> MDEAVGDLKQALPCVAESPTVHVEVHQRGSSTAKKEDINLSVRKLLNRHNIVFGDYTWTEFDEPFLTRNVQSVSIIDTELKVKDSQPIDLSACTVALHIFQLNEDGPSSENLEEETENIIAANHWVLPAAEFHGLWDSLVYDVEVKSHLLDYVMTTLLFSDKNVNSNLITWNRVVLLHGPPGTGKTSLCKALAQKLTIRLSSRYRYGQLIEINSHSLFSKWFSESGKLVTKMFQKIQDLIDDKDALVFVLIDAVESLTAARNACRAGTEPSDAIRVVNAVLTQIDQIKRHSNVVILTTSNITEKIDVAFVDRADIKQYIGPPSAAAIFKIYLSCLEELMKCQIIYPRQQLLTLRELEMIGFIENNVSKLSLL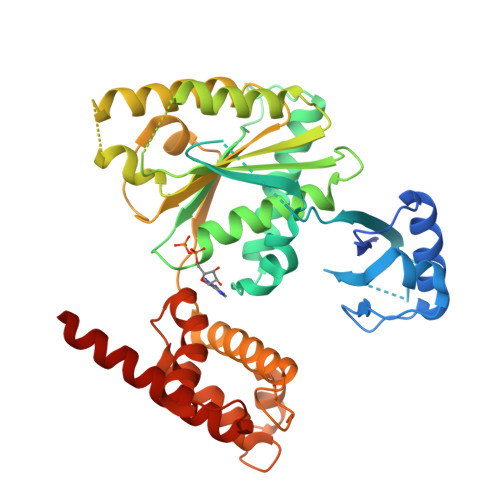LNDISRKSEGLSGRVLRKLPFLAHALYVQAPTVTIEGFLQALSLAVDKQFEERKKLAAYI An intriguing aspect of lymphocyte development is that the generation of a population of self-tolerant immune cells requires Ras activation by two distinct guanine nucleotide exchange factors, Ras guanine nucleotide releasing protein 1 (RasGRP1) and Son-of-Sevenless (SOS). To identify the structural basis for the regulation of RasGRP1, we have determined two crystal structures of RasGRP1. RasGRP1 is maintained in an autoinhibited, dimeric state, which is released by the coordinated binding of diacylglycerol and calcium second messenger molecules.

Residues 747–789 within the C-terminal region are predicted by the COILS webserver to contain a coiled coil and are spanned by the RasGRP1CC construct. We determined the crystal structure of RasGRP1CC at 1.6 Å resolution. Two molecules in the asymmetric unit of the crystal form a parallel, dimeric coiled coil of nearly 10 helical turns that is structurally similar to canonical coiled coil proteins such as GCN4. Leucine and isoleucine residues stabilize the dimer, and a pair of glutamine residues in the core maintains the proper sequence register between the two helices. Two pairs of ionic interactions (Glu 754-Lys 759′ and Glu 782-Lys 783′, where the primes refer to the second subunit in the dimer) further stabilize the dimer. The structure of the C-terminal coiled coil demonstrates that a second dimerization interface is present in RasGRP1. Consistent with this structure, RasGRP1CC is exclusively dimeric in solution from 30 μM to 1.5 mM monomer, based on multiangle light scattering measurements (data not shown). The fact that the C-terminal coiled coil is parallel and dimeric is consistent with an ability to readily connect with the autoinhibited catalytic module and reinforce formation of the C1-mediated dimer. Because coiled coil formation is independent of the C1-mediated interface, RasGRP1 is likely to remain dimeric upon disruption of the C1-mediated dimer by membrane binding. Dimerization in this way is expected to enhance the affinity of RasGRP1 for the membrane by allowing the dimer to engage two Ras molecules simultaneously.

>SELRHLRLPTYQELEQEINTLKADNDALKIQLKYAQKKIESLQLEKSNHVLAQMEQ[2x]>[6x]GSRMCGNNMSTPLPAIVPAARKATAAVIFLHGLGDTGHGWAEAFAGIRSSHIKYICPHAPVRPVTL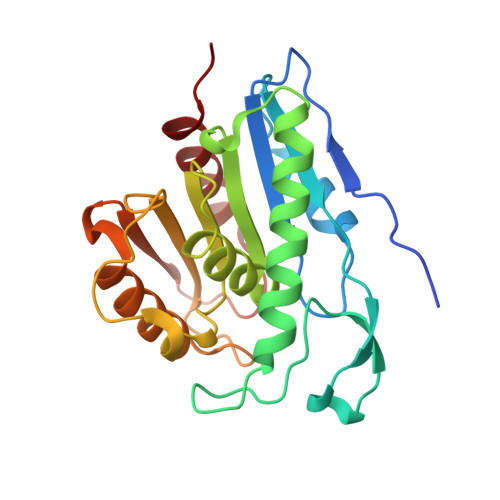NMNVAMPSWFDIIGLSPDSQEDESGIKQAAENIKALIDQEVKNGIPSNRIILGGFSQGGALSLYTALTTQQKLAGVTALSCWLPLRASFPQGPIGGANRDISILQCHGDCDPLVPLMFGSLTVEKLKTLVNPANVTFKTYEGMMHSSCQQEMMDVKQFIDKLLPPID> ATYDSA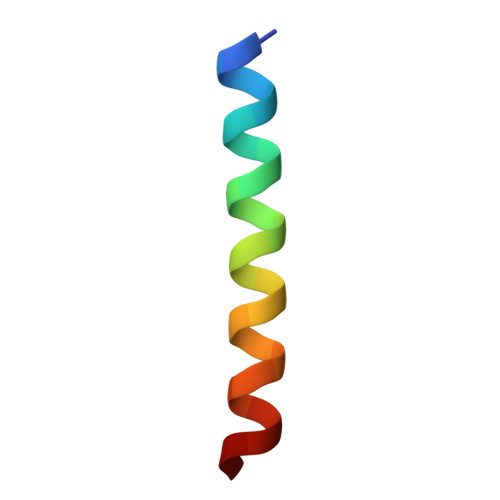LELVGQLNKVVDQLFEKAS> MGSDKIHHHHHHMIRPEYLRVLRKIYDRLKNEKVNWVVTGSLSFALQGVPVEV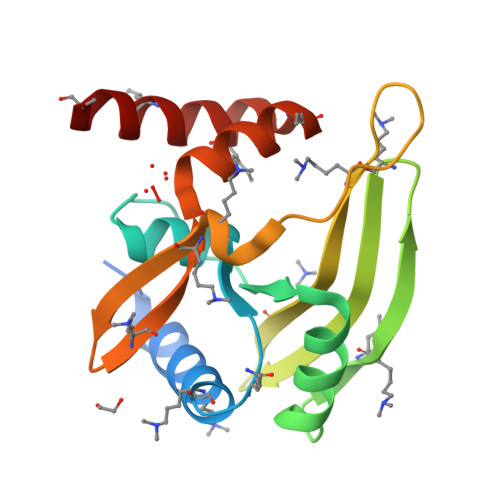HDIDIQTDEEGAYEIERIFSEFVSKKVRFSSTEKICSHFGELIIDGIKVEIMGDIRKRLEDGTWEDPVDLNKYKRFVETHGMKIPVLSLEYEYQAYLKLGRVEKAETLRKWLNERK> MLRIGRTLLAEVTTINSTTASVSGRLIRIRKKS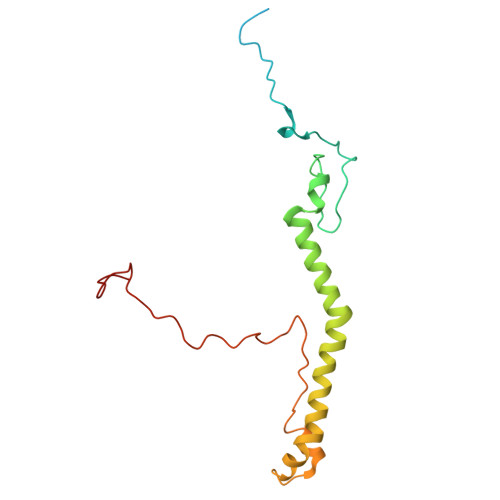KWIDRRSTRVPHNGKDIWYFGDQPSCALCHIRFRYKQDYEAHKESELHVNRLRWVETMNWWRETGEPAYLKASNEQWEWFEQHVLPTKAQEMGCTLDEARRVYRQAIMTETPTWHRPLQCPTVKQEVQEPRDQRWPASPKW> FAGLRQAV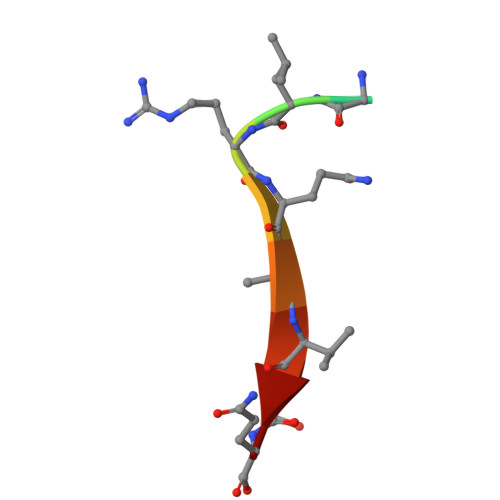TQ> PKITLLTLIKTAEHWARQDIRTIEDSKLRALLTLCAVMTRKFSKSQLSLLCETHLRREGLGQDQAEPVLEVYQRLHSDKGGSFEAALWQQWDRQSLIMFITAFLNIALQL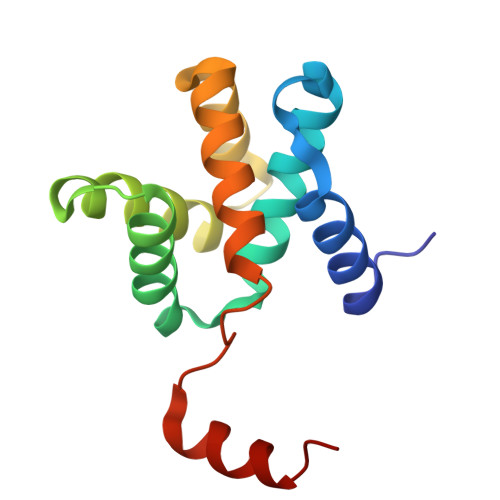PCESSAVVVSGLRTLVP> SMSRVLQAEELHEKALDPFLLQAEFFEIPMNFVDPKEYDIPGLVRKNRYKTILPNPHSRVCLTSPDPDDPLSSYINANYIRGYGGEEKVYIATQGPIVSTVADFWRMVWQEHTPIIVMITNIEEMNEKCTEYWPEEQVAYDGVEITVQKVIHTEDYRLRLISLKSGTEERGLKHYWFTSWPDQKTPDRAPPLLHLVREVEEAAQQEGPHCAPIIVHCSAGIGRTGCFIAT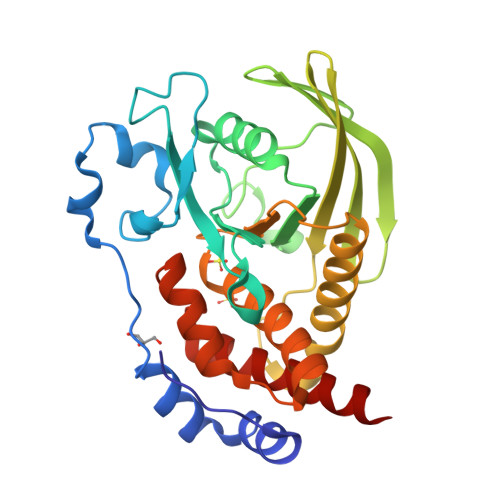SICCQQLRQEGVVDILKTTCQLRQDRGGMIQTCEQYQFVHHVMSLYEKQLSH> MGSSHHHHHHSSGLMDSLLGCGVSAAAREPVPRYLTSQPRVSEVAMQSAPLEQPAKRPRCDGSPRTPPSTPPATANLSADDDFQNTDLRTWEPEDVCSFLENRGFREKKVLDIFRDNKIAGSFLPFLDEDRLEDLGVSSLEERKKMIECIQQLSQSRIDLMKVFNDPIHGHIEFHPLLIRIIDTPQFQRLRYIKQLGGGYYVFPGASHNRFEHSLGVGYLAGCLVRALAEKQPELQISERDILCVQIAGLCRNLGHGPFSHMFDGRFIPRARPEKKWKHEQGSIEMFEHLVNSNELKLVMKNYGLVPEEDITFIKEQIMGPPITPVKDSLWPYKGRPATKSFLYEIVSNKRNGIDVDKWDYFARDCHHLGIQNNFDYKRFIKFARICEVEYKVKEDKTYIRKVKHICSREKEVGNLYDMFHTRNCLHRRAYQHKISNLIDIMITDAFLKADPYVEITGTAGKKFRISTAIDDMEAFTKLTDNIFLEVLHSTDPQLSEAQSILRNIECRNLYKYLGETQPKREKIRKEEYERLPQEVAKAKPEKAPDVELKAEDFIVDVINVDYGMEDKNPIDRVHFYCKSNSKQAVRINKEQVSQLLPEKFAEQLIRVYCKKKDGKSLDAAGKHFVQWCALRDFTKPQDGDIIAPLITPLKWNNKTSSCLQEVSKVKTCLKF

The sterile alpha-motif (SAM) and histidine-aspartate (HD) domain-containing protein 1 (SAMHD1) is a dNTP phosphohydrolase that restricts viral replication by limiting the cellular dNTP pool. The active tetramer form of SAMHD1 is induced by cellular nucleotides, which bind two allosteric sites of each subunit. The SAM domain is not required for dNTP hydrolysis and viral restriction by hSAMHD1, but is essential for these activities of mSAMHD1. To better understand the regulatory role of the SAM domain, we crystallized full-length mSAMHD1 in three different states (0, 1, and 2 allosteric nucleotides bound).

The 2-Allo structure was determined as a tetramer in I222 space group with one copy of the protein in each asymmetric unit of the crystal. The majority of the SAM and HD domains (residues 71–624) were built into the structure, although the C-terminal region including the reported phosphorylation site (T634)15,16,18,20 was not observed. Analysis of the 2-Allo structure in comparison to hHD structure reveals that the tetramer interface is fairly disordered with more than 25 residues unresolved. This full-length SAMHD1 structure captures the relationship between the SAM and HD domains, and shows that each SAM domain bridges three HD domains at the tetramer interface. Our 2-Allo mSAMHD1 structure shows that the SAM domain contributes to the formation of the allosteric site pocket by interacting with the HD domains to stabilize the allosteric nucleotides. Each allosteric site is formed as a deep cleft at the interface of HD domains from three subunits. Each SAM domain interacts intra- and inter-molecularly to contact the three HD domains, capping the nucleotides bound in the allosteric site pocket. At the inter-subunit interface, residues S566 and N567 of one HD domain interact across subunits with S142 and Q137 of the SAM domain from an adjacent mSAMHD1 molecule. At the mSAMHD1 intra-subunit interface, SAM domain residue R143 forms a salt bridge with HD domain residue E225 and the aromatic residues F109 and F112 from the SAM domain form stacking interactions with H161 and Y289 from the HD domain, respectively. Our 2-Allo mSAMHD1 structure shows that even this activated form of mSAMHD1 is still less compact than hSAMHD1, indicating an overall less stable tetramer.> SMDPEVTLLLQCPGGGLPQEQIQAELSPAHDRRPLPGGDEAITAIWETRLKAQPWLFDAPKFRLHSATLAPIGSRGPQLLLRLGLTSY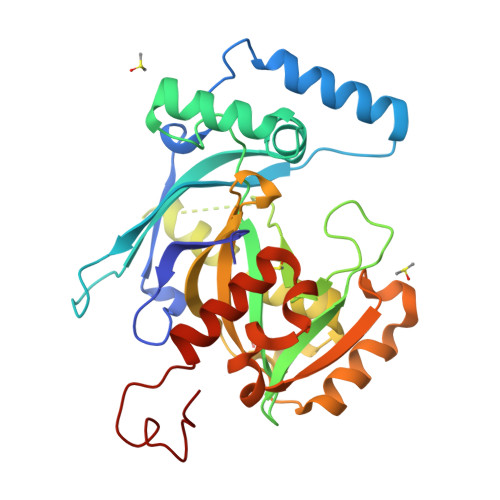RDFLGTNWSSSAAWLRQQGATDWGDTQAYLADPLGVGAALATADDFLVFLRRSRQVAEAPGLVDVPGGHPEPQALCPGGSPQHQDLAGQLVVHELFSSVLQEICDEVNLPLLTLSQPLLLGIARNETSAGRASAEFYVQCSLTSEQVRKHYLSGGPEAHESTGIFFVETQNVRRLPETEMWAELCPSAKGAIILYNRVQGSPTGAALGSPALLPPL> MVMGIFANCIFCLKVKYLPQQQKKKLQTDIKENGGKFSFSLNPQCTHIILDNADVLSQYQLNSIQKNHVHIANPDFIWKSIREKRLLDVKNYDPYKPLDI

pmcPARP4 is an ADP-ribosyltransferase (ART) that uses NAD+ as substrate to add ADP-ribose onto target proteins, a process called mono(ADP-ribosylation) or MARylation. PARP4 is also referred to as vault PARP since it can localize to the vault particle, a cytoplasmic ribonucleoprotein complex. PARP4 has a distinct domain composition relative to other PARP enzymes; however, the N-terminal region of PARP4 is homologous to a collection of domains found in PARP1, a regulator of multiple nuclear processes including the cellular response to DNA damage. Collectively, the study establishes the human PARP4 BRCT as a nucleic acid–binding module.

We determined a 1.75 Å crystal structure of the PARP4 BRCT domain that allowed us to compare its structure to other BRCT domains with nucleic acid–binding activity. The BRCT domain was crystallized using sitting drop vapor diffusion. Molecular replacement phasing of the diffraction data was realized using the AlphaFold predicted structure of PARP4 BRCT domain. Crystals of the BRCT domain diffracted to 1.75 Å and belong to space group F23 with one molecule in the asymmetric unit; the refined structure has a crystallographic R/RFREE of 0.175/0.188. However, there were several regions that required significant manual adjustments, and the final refined X-ray structure relative to the starting AlphaFold structure yielded an RMSD of 2.0 Å (comparing all 751 main chain and sidechain atoms). The major differences exist in loop regions connecting the core secondary structure elements, for example, the residues connecting strands β2 and β3 in the central beta-sheet. The general fold of the PARP4 BRCT resembles the structure of PARP1 BRCT domain, though the comparison shows some key differences in the positioning of residues that are important for PARP1 BRCT interaction with nucleic acid. The Thr420-Gly421-Thr422 motif in PARP1 is Ser38-Phe39-Ser40 in PARP4 and thus not highly conserved. Candidate regions were identified by examining the electrostatic surface potential for areas of concentrated positive charge that might engage the negatively charged backbone of nucleic acid. Indeed, the BRCT exhibited similar binding to each of the vtRNA, indicating that the BRCT domain alone is capable of mediating nucleic acid interaction.> VGSLNCIVAVSQNMGIGKNGDLPWPPLRNEFRYFQRMTTTSSVEGKQNLVIMGKKTWFSIPERNRPLKGRINLVLSRELKEPPQGAH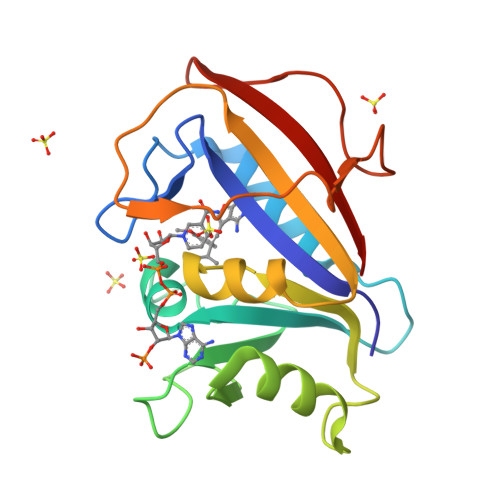FLSRSLDDALKLTEQPELANKVDMVWIVGGSSVYKEAMNHPGHLKLFVTRIMQDFESDTFFPEIDLEKYKLLPEYPGVLSDVQEEKGIKYKFEVYEKND>MGSSHHHHHHSSGRENLYFQGMELLKHLSQRQYIDGEWVESANKNTRDIINPYNQEVIFTVSEGTKEDAERAILAARRAFESGEWSQETAETRGKKVRAIADKIKEHREALARLETLDTGKTLEESYADMDDIHNVFMYFAGLADKDGGEMIDSPIPDTESKIVKEPVGVVTQITPWNYPLLQASWKIAPALATGCSLVMKPSEITPLTTIRVFELMEEVGFPKGTINLILGAGSEVGDVMSGHKEVDLVSFTGGIETGKHIMKNAANNVTNIALELGGKNPNIIFDDADFELAVDQALNGGYFHAGQVCSAGSRILVQNSIKDKFEQALIDRVKKIKLGNGFDADTEMGPVISTEHRNKIESYMDVAKAEGATIAVGGKRPDRDDLKDGLFFEPTVITNCDTSMRIVQEEVFGPVVTVEGFETEQEAIQLANDSIYGLAGAVFSKDIGKAQRVANKLKLGTVWINDFHMLFAQAPW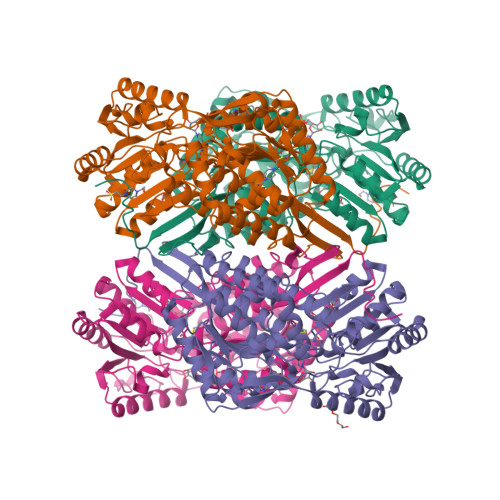GGYKQSGIGRELGKEGLEEYLVSKHILTNTNPQLVNWFSK[4x]>CPRFLKVKNWETDVVLTDTLHLKSTLETGCTEHICMGSIMLPSQLTRKPEDVRTKDQLFPLAKEFLDQYYSSIKRFGSKAHMDRLEEVNKEIESTSTYQLKDTELIYGAKHAWRNASRCVGRIQWSKLQVFDARD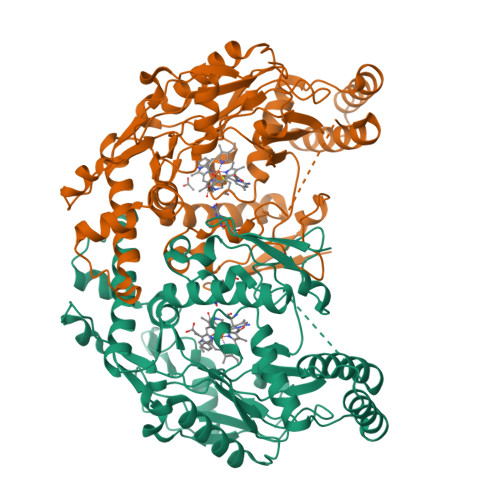CTTAHGMFNYICNHVKYATNKGNLRSAITIFPQRTDGKHDFRVWNSQLIRYAGYKQPDGSTLGDPANVQFTEICIQQGWKAPRGRFDVLPLLLQANGNDPELFQIPPELVLEVPIRHPKFDWFKDLGLKWYGLPAVSNMLLEIGGLEFSACPFSGWYMGTEIGVRDYCDNSRYNILEEVAKKMDLDMRKTSSLWKDQALVEINIAVLYSFQSDKVTIVDHHSATESFIKHMENEYRCRGGCPADWVWIVPPMSGSITPVFHQEMLNYRLTPSFEYQPDPWNTHVWKG[2x]> MDAAAS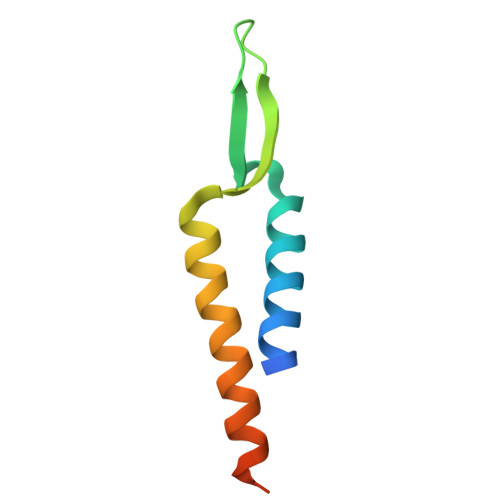ATETATRDQLTKEAFQNPDNQKVNIDELGNAIPSGVLKDDVVANIEEQAKAAGEEAKQQAIENLEHHHHHH>GSMSVYRFEDKTPAVHPTAFIAPGAYVVGAVEVGEGASIWFGAVVRGDLERVVVGPGTNVQDGAVLHADPGFPCLLGPEVTVGHRAVVHGAVVEEGALVGMGAVVLN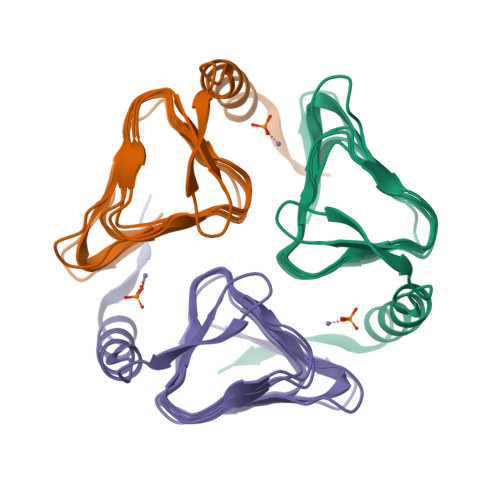GARIGKNAVVGAGAVVPPGMEVPEGRLALGVPARVVRPIDPPGNAPRYRALAERYRKALFPVAT[6x]Peptidyl dipeptidase A is a highly glycosylated ectoenzyme that cleaves dipeptides from the C-terminus of a broad range of oligopeptides. AnCE is a single-domain glycosylated protein that closely shares enzymatic properties with human ACE (in particular the C-domain of human somatic ACE) and is inhibited by classic inhibitors of the human enzymes 14–17. In this study, we elucidate how the natural peptides Ang II (the principal end-product of the renin-angiotensin–aldosterone system), Arg–Pro–Pro (the BK-derived peptide) and bradykinin-potentiating peptide-b (BPPb, a snake venom inhibitor) bind to the active site of AnCE, revealing novel interactions involving several enzyme subsites. Comparison of the four structures clearly shows a common mode of peptide binding to AnCE.

Therefore, it was not surprising that the structures of AnCE in complex with BK and Thr6–BK showed Arg–Pro–Pro bound in a similar fashion in the active site cleft. Strong hydrogen bond interactions with AnCE anchor the main chain of the N-terminal Arg (P1) at the S1 site (His367, His371 and Tyr507), which is also involved in coordination with the zinc ion. Furthermore, the side chain for this residue is stabilized through contact with Tyr496. Additionally, both structures bind a citrate ion (from the crystallization medium) at the same position, making contact with the N-terminus of the bound BK (1-3) peptide. The citrate ion also interacts directly with the AnCE main chain and the surrounding water molecules. The two Pro residues at positions P1′ and P2′ form a strong interaction with AnCE through hydrogen bonds with residues His497, His337 and Tyr504, Lys495 respectively. The general mode of binding for BK (1-3) appears similar to that of Ang II, particularly through the various hydrogen bonds with AnCE. Experimental evidence suggests a preferred affinity for Pro at the S2′ binding site and highlights the importance of the hydrophobic pocket (formed by residues Phe441, Phe511, Tyr504 and Tyr507) for peptide recognition, which allows the products of BK and Thr6–BK hydrolysis to shift position and ‘register’ in the active site subsites. In both cases, complete hydrolysis of the peptide to the end point resulted in clear visible electron density for the tripeptide (Arg–Pro–Pro) in their respective crystal structures.

> ALVKEEIQAKEYLENLNKELAKRTNVETEAAWAYGSNITDENEKKKNEISAELAKFMKEVASDTTKFQWRSYQSEDLKRQFKALTKLGYAALPEDDYAELLDTLSAMESNFAKVKVCDYKDSTKCDLALDPEIEEVISKSRDHEELAYYWREFYDKAGTAVRSQFERYVELNTKAAKLNNFTSGAEAWLDEYEDDTFEQQLEDIFADIRPLYQQIHGYVRFRLRKHYGDAVVSETGPIPMHLLGNMWAQQWSEIADIVSPFPEKPLVDVSAEMEKQGYTPLKMFQMGDDFFTSMNLTKLPQDFWDKSIIEKPTDGRDLVCHASAWDFYLTDDVRIKQCTRVTQDQLFTVHHELGHIQYFLQYQHQPFVYRTGANPGFHEAVGDVLSLSVSTPKHLEKIGLLKDYVRDDEARINQLFLTALDKIVFLPFAFTMDKYRWSLFRGEVDKANWNCAFWKLRDEYSGIEPPVVRSEKDFDAPAKYHISADVEYLRYLVSFIIQFQFYKSACIKAGQYDPDNVELPLDNCDIYGSAAAGAAFHNMLSMGASKPWPDALEAFNGERIMSGKAIAEYFEPLRVWLEAENIKNNVHIGWTTSNKCVS;> RPPGFSPFR2-methyl-5-phenyl-1H-pyrrole-3-carboxamide | C12 H12 N2 O | 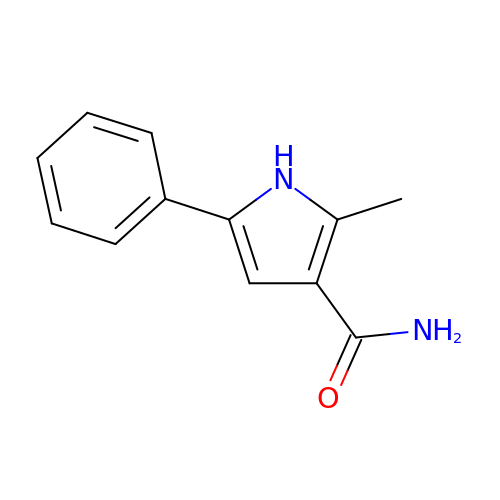CJXRIVBNRCQKLJ-UHFFFAOYSA-N>MGHHHHHHHHSSGHIEGRHMAHLLIVNVASHGLILPTLTVVTELVRRGHRVSYVTAGGFAEPVRAAGATVVPYQSEIIDADAAEVFGSDDLGVRPHLMYLRENVSVLRATAEALDGDVPDLVLYDDFPFIAGQLLAARWRRPAVRLSAAFASNEHYSFSQDMVTLAGTIDPLDLPVFRDTLRDLLAEHGLSRSVVDCWNHVEQLNLVFVPKAFQIAGDTFDDRFVFVGPCFDDRRFLGEWTRPADDLPVVLVSLGTTFNDRPGFFRDCARAFDGQPWHVVMTLGGQVDPAALGDLPPNVEAHRWVPHVKVLEQATV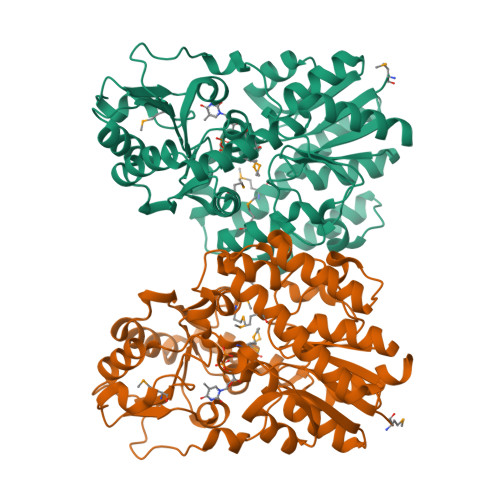CVTHGGMGTLMEALYWGRPLVVVPQSFDVQPMARRVDQLGLGAVLPGEKADGDTLLAAVGAVAADPALLARVEAMRGHVRRAGGAARAADAVEAYLARAR[2x]> MTQAWLWIGVISMALGSVFFGFGAHNAKNERWQILYTLNFFICLIAAGLYLAMALGLGVNVINGRPTYWVRFVTWFCSTPLLLLDLTFLGRTSLPLTGSLLGANAYMLVTGFVATVTPKPMSYIWYI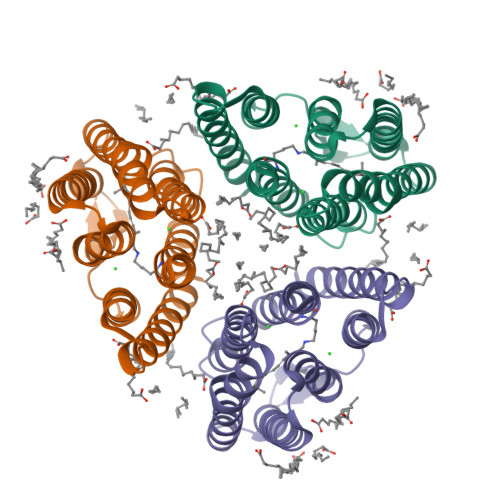VSCAAYLAIVYLLAQPYRIAAERKHPRSKQAFRTLVTVHLVLWTLYPIVWILSPEGFSTFTQGSETMFYTLLDIASKVGFGFLSLNTLHTLEQATEPARETHLSY>[2x]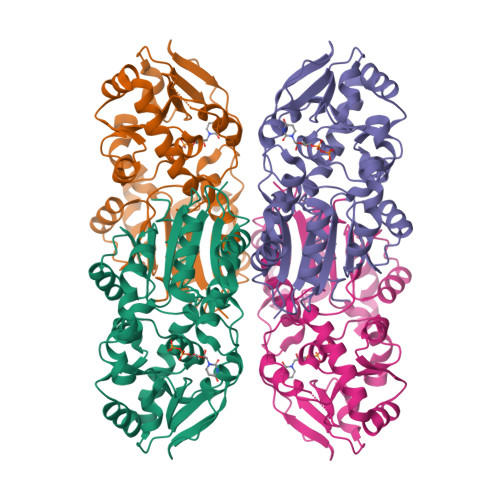SEFELRRQACMRVYITNINGQSIQSTAQLCQNTVTDVAVSLGYRELGIYCYQIHTDSESELSKRLDGIVAGLRHGDVVIFQTPTWNTTEFDEKLMNKLKLYDIKIVLFIHDVVPLMFSGNFYLMDRTIAYYNKADVVVAPSQKMIDKLRDFGMNVSKTVVQGMWDHPTQAPMFPAGLKREIHFPGNPERFSFVKEWKYDIPLKVYTWQNVELPQNVHKINYRPDEQLLMEMSQGGFGLVWMDDKDKEYQSLYCSYKLGSFLAAGIPVIVQEGIANQELIENNGLGWIVKDVEEAIMKVKNVNEDEYIELVKNVRSFNPILRKGFFTRRLLTESVFQAIC>[2x]PGLMLDYNLNG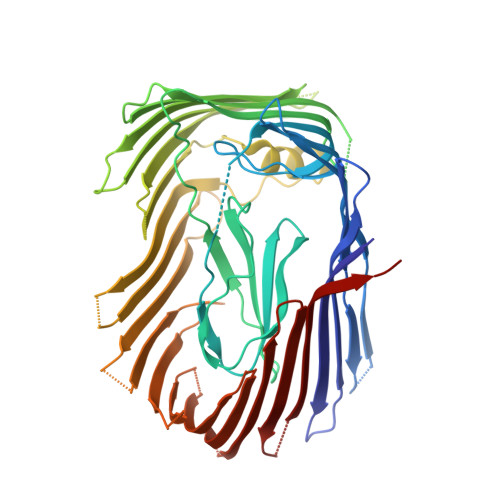TVSRNYQGGDSHQFSYNGTVGGNLGPWRLRADYQGSQEQSRYNGEKTTNRNFTWSRFYLFRAIPRWRANLTLGENNINSDIFRSWSYTGASLESDDRMLPPRLRGYAPQITGIAETNARVVVSQQGRVLYDSMVPAGPFSIQDLDSSVRGRLDVEVIEQNGRKKTFQVDTASVPYLTRPGQVRYKLVSGRSRGYGHETEGPVFATGEASWGLSNQWSLYGGAVLAGDYNALAAGAGWDLGVPGTLSADITQSVARIEGERTFQGKSWRLSYSKRFDNADADITFAGYRFSERNYMTMEQYLNARYRNDYSSREKEMYTVTLNKNVADWNTSFNLQYSRQTYWDIRKTDYYTVSVNRYFNVFGLQGVAVGLSASRSKYLGRDNDSAYLRISVPLGTGTASYSGSMSNDRYVNMAGYTDTFNDGLDSYSLNAGLNSGGGLTSQRQINAYYSHRSPLANLSANIASLQKGYTSFGVSASGGATIT> DSYTHLSFYEKRELFRKKLREIEGPEVTLVNEVDDEPCPSLDFQFISQYRLTQGVIPPDPNAQSGCNCSSLGGCD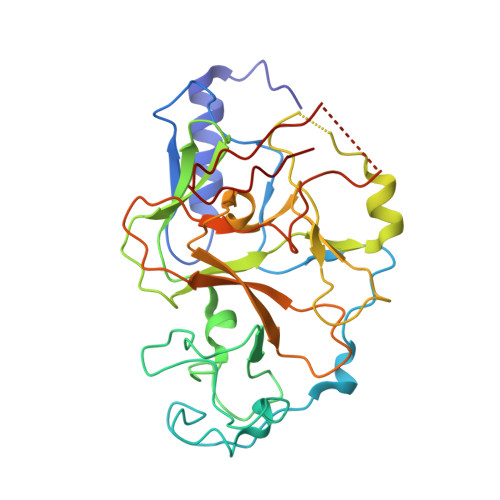LNNPSRCECLDDLDEPTHFAYDAQGRVRADTGAVIYECNSACSCSMECPNRVVQRGRTLPLEIFKTKEKGWGVRSLRFAPAGTFITCYLGEVITSAEAAKRDKNYDDDGITYLFDLDMFDDASEYTVDAQNYGDVSRFFNHSCSPNIAIYSAVRNHGARTIYDLAFFAIKDIQPLEELTFDYAGAKDFSPVQSQKSQQNRISKLRRQCKCGSANCRGWLFG>[2x]MADPWQECMDYAVTLARQAGEVVCEAIKNEMNVMLKSSPVDLVTATDQKVEKMLISSIKEKYPSHSFIGEESVAAGEKSILTDNPTWIIDPIDGTTNFVHRFPFVAVSIGFAVNKKIEFGVVYSCVEGKMYTARKGKGAFCNGQKLQVSQQEDITKSLLVTELGSSRTPETVRMVLSNMEKLFC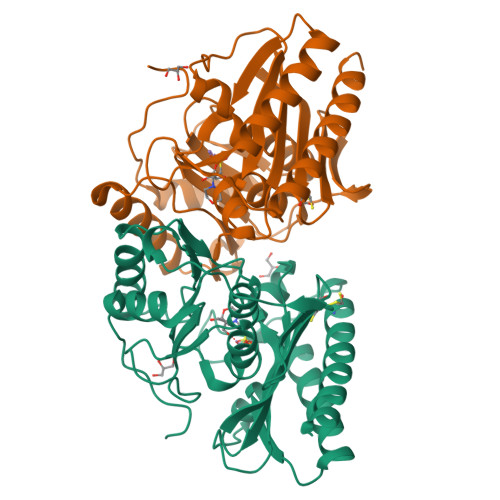IPVHGIRSVGTAAVNMCLVATGGADAYYEMGIHCWDVAGAGIIVTEAGGVLMDVTGGPFDLMSRRVIAANNRILAERIAKEIQVIPLQRDDED PNP (PNP: E.C. 2.4.2.1) catalyzes the reversible phosphorolysis of N-ribosidic bonds of nucleosides and generates a purine base and ribose-1- phosphate. The homotrimeric class enzymes utilize 6-oxopurines as substrates, while the homohexameric class enzymes utilize 6-oxopurines and 6-aminopurines. In the present study, we report the structural and biochemical characterization of K. lactis PNP (KlacPNP). Based on the observed oligomeric state in solution, KlacPNP can be classified in the low molecular mass, homotrimeric class of NP-I family of nucleoside phosphorylases.

We report the crystal structure of KlacPNP at 1.97 Å resolution and observed an extra electron density at the active site. There were three molecules in the asymmetric unit, corresponding to one biological trimer of KlacPNP. All three monomers assembled to form a trimer having a non-crystallographic, 3-fold symmetry. The most distinguishing feature of KlacPNP is the presence of a long loop connecting β9 and α7, which participates extensively in establishing intermolecular interactions. A catalytic site is formed in the vicinity of the intersubunit interface, where Phe172 from adjacent monomer participates in the formation of an active site pocket. Based on the observed mass, we could unambiguously identify the bound ligand as hypoxanthine. Hypoxanthine remained bound to the protein throughout the protein purification steps and crystallization process, suggesting high affinity of hypoxanthine to KlacPNP. In addition to five potential hydrogen bonds between protein and hypoxanthine, two indirect water-mediated interactions are also observed. In addition to hydrogen bonds, π-π interactions mediated by the Phe213 side chain, lying almost perpendicular to the planar ring of the ligand, are also present. Similarly, in the crystal structure of KlacPNP, the structurally equivalent Asn256 forms the hydrogen bond with O6 of hypoxanthine, which is an end-product of inosine phosphorolysis.

>[3x]MSSLDINEQRALIKSAHRYISEKLEDHFSSEFLPKALVICGSGLSGISTKIADEPKPLILSYSTIPGFKVSTVPGHSGELIFGYMNGAPVVLMNGRLHSYEGHSLAETVHPIRALHLLGSINVLIVTNAAGGINASFKAGDLMCVYDHINFPGLCGFHPLRGANFDEFGPRFLATSDAYDLELRKLLFSKKKELNIERKIHEGTYSYVHGPTFESRAESRFLRLAGTDAVGMSTVPEVVTARHCGWRVLALSLITNECVVDPPASAHDENPVPIQEGKATHEEVLENSAKASKDVQELIFSVVAEIHHHHHH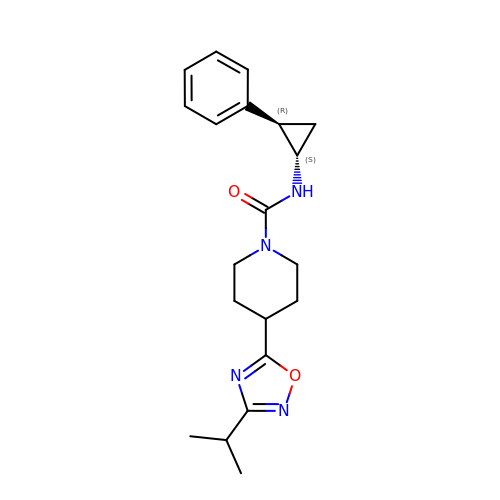4-[3-(1-methylethyl)-1,2,4-oxadiazol-5-yl]-N-[(1S,2R)-2-phenylcyclopropyl]piperidine-1-carboxamide | C20 H26 N4 O2 | WYQYSMZPAAVISB-SJORKVTESA-N>MILMRRTLKAAILGATGLVGIEYVRMLSNHPYIKPAYLAGKGSVGKPYGEVVRWQTVGQVPKEIADMEIKPTDPKLMDDVDIIFSPLPQGAAGPVEEQFAKEGFPVISNSPDHRFDPDVPLLVPELNPHTISLIDEQRKRREWKGFIVTTPLCTAQGA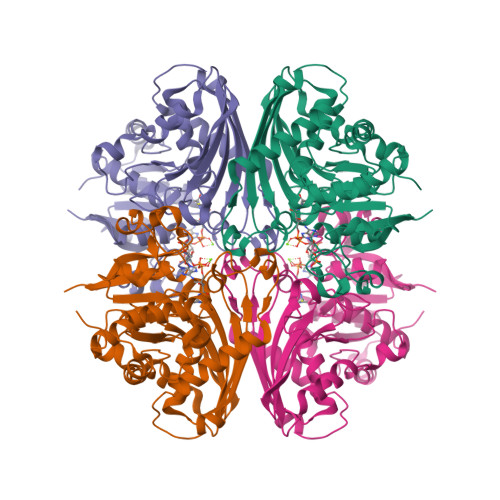AIPLGAIFKDYKMDGAFITTIQSLSGAGYPGIPSLDVVDNILPLGDGYDAKTIKEIFRILSEVKRNVDEPKLEDVSLAATTHRIATIHGHYEVLYVSFKEETAAEKVKETLENFRGEPQDLKLPTAPSKPIIVMNEDTRPQVYFDRWAGDIPGMSVVVGRLKQVNKRMIRLVSLIHNTVRGAAGGGILAAELLVEKGYIEK[6x]ABCG2 transports uric acid and plays an essential role in the pathology of gout, but also confers resistance to a variety of chemotherapeutics including topoisomerase inhibitors (i.e., mitoxantrone (MXN), etoposide, topotecan, SN38), anthracyclines (i.e., doxorubicin and daunorubicin), antimetabolites (i.e., methotrexate and 5-fluorouracil), and photosensitizers (i.e., pheophorbide A). There are more than 200 known ABCG2 substrates which have highly diverse chemical structures and functions, and the substrate spectrum of ABCG2 is substantially overlapping with and yet distinct from that of Pgp or ABCC14. In this work, we used cryo-EM and biochemical assays to characterize the structures of ABCG2 in the unliganded state, and in the presence of the chemotherapeutic agents imatinib, MXN, or SN38. In total, our results delineate a new paradigm for the conformational transition cycle of ABCG2, and reveal how different chemotherapy compounds distinctively alter the conformational space of the transporter.

The structure of ABCG2 bound to imatinib was determined in the same fashion as the apo-closed conformation, except that the nanodisc reconstituted transporter was incubated with imatinib on ice for ~45 min before plunge freezing cryo-EM grids. Three-dimensional (3D) classification of ABCG2 particles bound to imatinib demonstrated a single predominant conformation with the TM helices in an inward open facing conformation. The inward open conformation observed in the presence of imatinib is essentially identical to the conformation seen previously with ABCG2 bound to 5D3 Fab fragments or high affinity inhibitors. The final cryo-EM structure of imatinib-bound ABCG2 at an overall resolution of 4.0 Å revealed one imatinib molecule bound in the inward-facing cavity between ABCG2 monomers. Imatinib bound in a location that spans across the top of the inward-facing cavity just beneath the leucine plug, similar to the previous binding position of the transport substrate E1S and the inhibitor MB136. Imatinib is sandwiched via π-stacking interactions between the Phe439 phenyl moiety from opposing ABCG2 monomers. Although bound in a similar location as previously seen with the inhibitor MB136, imatinib occupies significantly less volume at the dimer interface. Moreover, imatinib is bound relatively high in the inward facing cavity, whereas inhibitors such as MB136 and MZ29 extend farther towards the cytosol and make additional contacts with TM1. Although imatinib occupies a smaller volume and makes fewer protein contacts than other ABCG2 inhibitors, the molecule similarly acts like a wedge to force ABCG2 into the inward facing conformation and ultimately prevent ATP hydrolysis. Thus, in the presence of transport substrates MXN or SN38 a significant fraction of ABCG2 particles appear not to bind the substrates and remain in the apo-closed conformation.

>[2x]MSSSNVEVFIPVSQGNTNGFPATASNDLKAFTEGAVLSFHNICYRVKLKSGFLPCRKPVEKEILSNINGIMKPGLNAILGPTGGGKSSLLDVLAARKDPSGLSGDVLINGAPRPANFKCNSGYVVQDDVVMGTLTVRENLQFSAALRLATTMTNHEKNERINRVIQELGLDKVADSKVGTQFIRGVSGGERKRTSIGMELITDPSILFLDEPTTGLDSSTANAVLLLLKRMSKQGRTIIFSIHQPRYSIFKLFDSLTLLASGRLMFHGPAQEALGYFESAGYHCEAYNNPADFFLDIINGDSTAVALNREEDFKATEIIEPSKQDKPLIEKLAEIYVNSSFYKETKAELHQLSGGEKKKKITVFKEISYTTSFCHQLRWVSKRSFKNLLGNPQASIAQIIVTVVLGLVIGAIYFGLKNDSTGIQNRAGVLFFLTTNQCFSSVSAVELFVVEKKLFIHEYISGYYRVSSYFLGKLLSDLLPMRMLPSIIFTCIVYFMLGLKPKADAFFVMMFTLMMVAYSASSMALAIAAGQSVVSVATLLMTICFVFMMIFSGLLVNLTTIASWLSWLQYFSIPRYGFTALQHNEFLGQNFCPGLNATGNNPCNYATCTGEEYLVKQGIDLSPWGLWKNHVALACMIVIFLTIAYLKLLFLKKYS6-(1,4,5,6-tetrahydropyrimidin-2-yl)-2-[4'-(1,4,5,6-tetrahydropyrimidin-2-yl)biphenyl-4-yl]-1H-indole 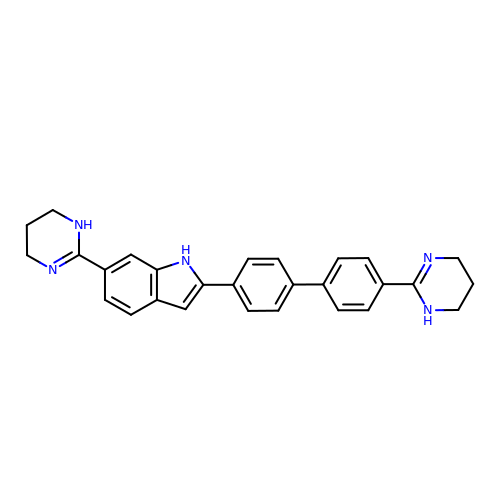| C28 H27 N5 | VZIHOYLEOYSFAG-UHFFFAOYSA-N> GHMGAASASLAIGGVVIIGGGGHAKVVIESLRACGETVAAIVDADPTRRAVLGVPVVGDDLALPMLREQGLSRLFVAIGDNRLRQKLGRKARDHGFSLVNAIHPSAVVS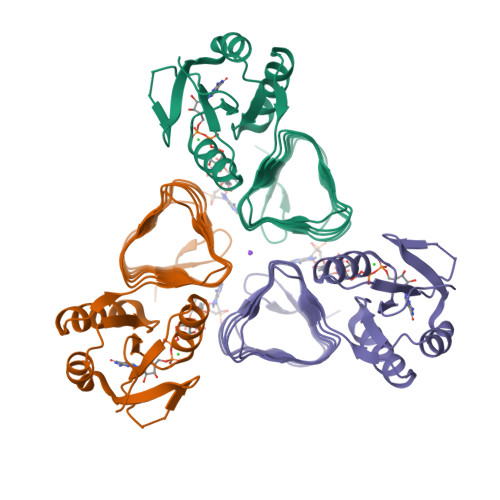PSVRLGEGVAVMAGVAINADSWIGDLAIINTGAVVDNDCRLGAACHLGPASALAGGVSVGERAFLGVGARVIPGVTIGADTIVGAGGVVVRDLPDSVLAIGVPAKIKGDRS> MSGIGALFRPLPRMGPRLPFELPAPPRPHLPMPAPRPLPRPAPGALTLSRDRTREAERDCSKSQGRDKDCVECPPSRGEMAIANNGKGHSMSDLSARYQQWVTNFPFPHEWFWSGTWWDGFDEPRCTLLEAKANYAFLFVPLLGVPRPWARAKVKSDLLQKAEVHSDKARPTPPVFVEWHFLQRIVYEYCAA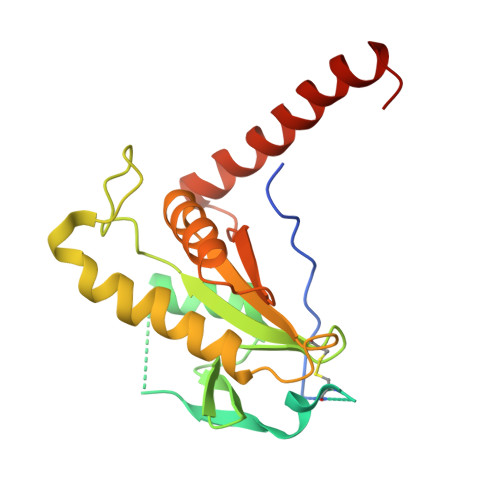EYLRMGLANLKAFWNPMPGTDEHDDYQETRAKEQEEMKRFCEENPGYCA>LMGDDKVKKEVGRASWKYFHTLLARFPDEPTPEEREKLHTFIGLYAELYPCGECSYHFVKLIEKYPVQTSSRTAAAMWGCHIHNKVNEYLKKDIYDCATILEDYD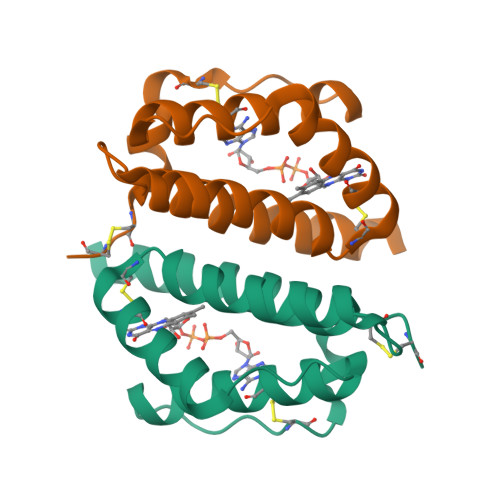CGCSDSDGKRVS[4x]>[21x]MAKLETVTLGNIGKDGKQTLVLNPRGVNPTNGVASLSQAGAVPALEKRVTVSVSQPSRNRKN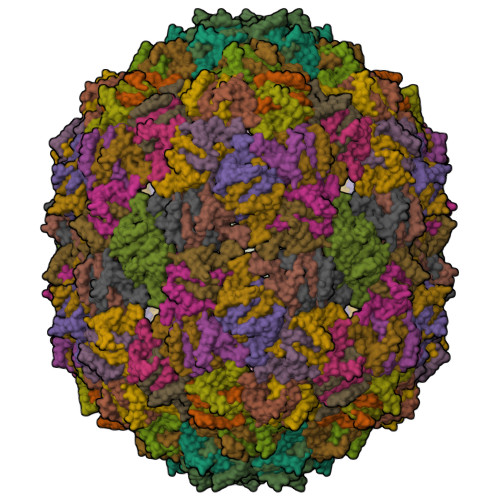YKVQVKIQNPTACTANGSCDPSVTRQAYADVTFSFTQYSTDEERAFVRTELAALLASPLLIDAIDQLNPAY>TDLPRPSISAEPGTVIPLGSHVTFVCRGPVGVQTFRLERERNYLYSDTEDVSQTSPSESEARFRIDSVNAGNAGLFRCIYYKSRKWSEQSDYLELVVK[2x];>VTAKELAEKAGAAAGLKAGDIHGMKIVIEGLKALKVDTLKSGIFNSFVQNSHYTEVTGLAIAIDTEMNEVCSATYIGIHPICVVREKLGVIPKAGGTMVKQKDAITNVLKQALEKATQSAEALSETTAEDVAAKLTAQKTGAINT[2x]

RIFIN, a large family of Plasmodium variant surface antigens, plays a crucial role in malaria pathogenesis by mediating immune suppression through activation of inhibitory receptors such as LAIR1, and antibodies with LAIR1 inserts have been identified that bind infected erythrocytes through RIFIN. RIFIN also mediates immune suppression through activation of inhibitory immune receptors including leukocyte-associated immunoglobulin-like receptor 1 (LAIR1) and leukocyte immunoglobulin-like receptor B1 (LILRB1). Notably, human monoclonal antibodies that contain LAIR1-domain insertions in either switch region or between V and DJ regions have been isolated from donors, who have had malaria. To define the structural basis underpinning interactions between wild-type and antibody-inserted LAIR1 and polymorphic RIFIN, we investigated the overall architecture of three types of LAIR1-inserted antibodies, determined crystal structures of LAIR1 in complex with the RIFIN-interactive regions from two RIFINs (PF3D7_1040300 and PF3D7_0401300), and used the resultant structural information to derive a LAIR1-binding signature and to identify RIFINS from diverse Plasmodium species capable of recognizing LAIR1.

To facilitate structural determination of the RIFIN-V2-LAIR1 interaction, we took advantage of the affinity maturation of the LAIR1 ectodomain from antibody MGD21, which increases its affinity to RIFIN (PF3D7_1040300) to 6.2 nM, from lower than 1 µM. The crystal structure of the RIFIN V2 (PF3D7_1040300) in complex with LAIR1 extended to 2.7-Å resolution, while negative-stain (ns)-EM 3D reconstruction of the MGD21 Fab complex with RIFIN V2 (PF3D7_1400600) indicated the Fab region not to be involved in RIFIN binding. The RIFIN-V2-LAIR1 complex resembled a razor with an exchangeable cartridge, where RIFIN V2 is the “handle” and LAIR1 is the “cartridge”. The RIFIN-V2 portion of the complex comprised 6 helices (α1-α6). Two longer helices, α1 and α6, and two shorter helices, α3 and α4, formed a four-helix bundle with helices α2 and α5 packed perpendicularly to the bundle. Helix α5 and its adjacent loops (α4-α5 and α5-α6) were connected by a disulfide bond (C254-C265) between α4 and α5; this region (hereafter referred to as the apex region) is likely located distally from the membrane, as the carboxyl terminus of the V2 region connects directly to the transmembrane. Comparison to the previously determined structure of ligand-free LAIR1 (PDB 3KGR11) suggested the binding of RIFIN to induce conformational alterations in the C-C’ loop, although their overall structures were essentially identical with a root-mean-square deviation (rmsd) of 0.41 Å over all Cα atoms. Interestingly, the interface between RIFIN-V2 and LAIR1 buried a surface area of 917 Å2 on each protein. The interface consisted of backbone-mediated hydrogen bonds and extensive hydrophobic interactions with highly complementary shapes matching between RIFIN and LAIR1.> MDKKSLYKYLLLRSTGDMHRAKSPTIMTRVTNNVYLGNYKNAMDAPSSEVKFKYVLNLTMDKYTLPNSNINIIHIPLVDDTTTDISKYFDDVTAFLSKCDQRNEPVLVHCVAGVNRSGAMI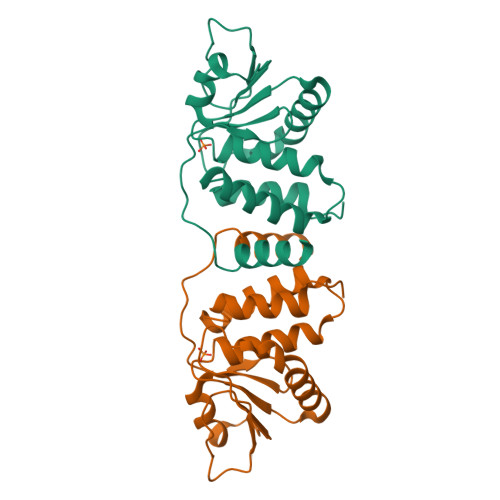LAYLMSKNKESSPMLYFLYVYHSMRDLRGAFVENPSFKRQIIEKYVIDKN> MGVNAVHWFRKGLRLHDNPALKECIQGADTIRCVYILDPWFAGSSNVGINRWRFLLQCLEDLDANLRKLNSRLFVIRGQPADVFPRLFKEWNITKLSIEYDSEPFGKERDAAIKKLATEAGVEVIVRISHTLYDLDKIIELNGGQPPLTYKRFQTLVSKMEPLEMPADTITSDVIGKCMTPLSDDHDEKYGVPSLEELGFDTDGLSSAVWPGGETEALTRLERHLERKAWVANFERPRMNANSLLASPTGLSPYLRFGCLSCRLFYFKLTDLYKKVKKNSSPPLSLYGQLLWREFFYTAATNNPRFDKMEGNPICVQIPWDKNPEALAKWAEGRTGFPWIDAIMTQLRQEGWIHHLARHAVACFLTRGDLWISWEEGMKVFEELLLDADWSINAGSWMWLSCSSFFQQFFHCYCPVGFGRRTDPNGDYIRRYLPVLRGFPAKYIYDPWNAPEGIQKVAKCLIGVNYPKPMVNHAEASRLNIERMKQIYQQL;> GAMDP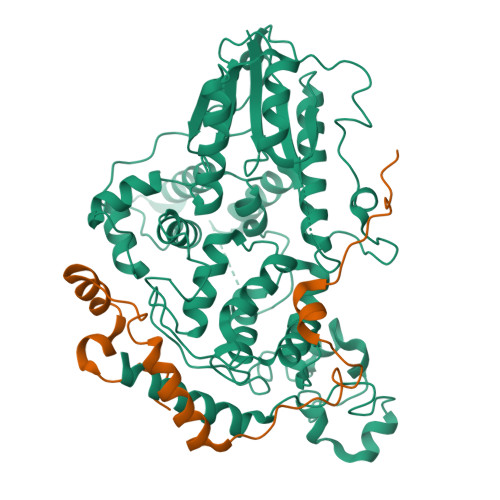EFSSDTSHTSKYFGSIDSSENNHKAKMNTGMEESEHFIKCVLQDPIWLLMADADSSVMMTYQLPSRNLEAVLKEDREKLKLLQKLQPRFTESQKQELREVHQWMQTGGLPAAIDVAECVYCES4-(isoquinolin-1-yl)-N-[2-(morpholin-4-yl)ethyl]benzamide | C22 H23 N3 O2 | 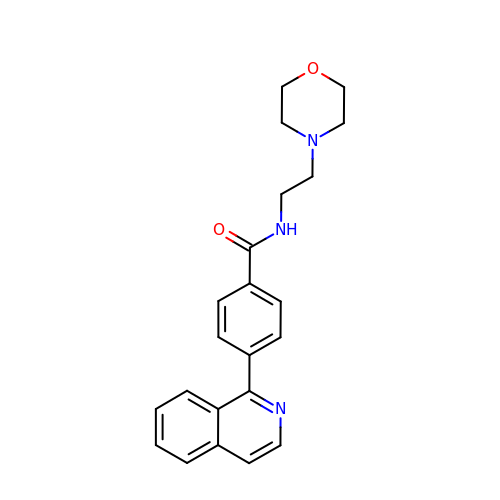JZHDIGBWZULPFR-UHFFFAOYSA-N>GGSMSNPDYCIPNFSQTVNERTIIDIFTICRYRSPLVVFCLSHNELAKKYAQDVSMSSGTHVHIIDGSVEITVSLYRTFRTIATQLLGRMQIVVFVTVDKSVVSTQVMKSIAWAFRGSFVELRNQSVDSSTLVSKLENLVSFAPLYNVPKCGPDYYGPTVYSELLSLATNARTHWYATIDYSMFTRSVLTGFVAKYFNEEAVPIDKRIVSIVGYNPPYVWTCLRHGIRPTYIEKSLPNPGGKGPFGLILPVINELVLKSKVKYVMHNPQIKLLCLDTFMLSTSMNILYIGAYPATHLLSLQLNGWTILAFDPKITSDWTDAMAKATGAKVIGVSKEFDFKSFSVQANQLNMFQNSKLSVIDDTWVETDYEKFQSEKQAYFEWLIDRTSIDVRLISMKWNRSKDTSVSHLLALLPQPYGASIREMRAFFHKKGASDIKILAAETEKYMDDFTAMSVSDQINTQKFMHCMITTVGDALKMDLDGGRAVIASYSLSNSSNSKERVLKFLSDANKAKAMVVFGAPNTHRLAYAKKVGLVLDSAIKMSKDLITFSNPTGRRWRDYGYSQSELYDAGYVEITIDQMVAYSSDVYNGVGYFA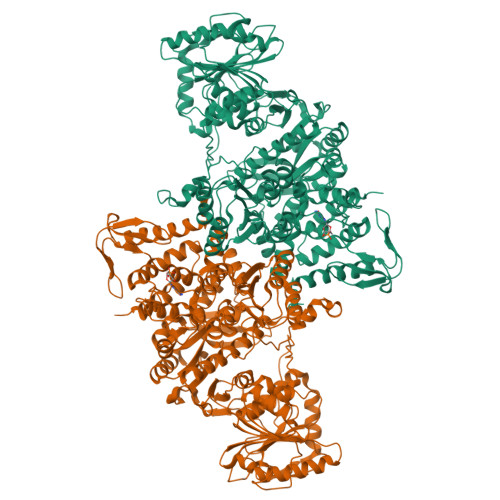NSTYNDLFSWYIPKWYVHKRMLMQDIRLSPAALVKCFTTLIRNICYVPHETYYRFRGILVDKYLRSKNVDPSQYSIVGSGSKTFTVLSHFEVPHECGPLVFEASTDVNISGHLLSLAIAAHFVASPMILWAEQMKYMAVDRMLPPNLDKSLFFDNKVTPSGALQRWHSREEVLLAAEICESYAAMMLNNKHSPDIIGTLKSAINLVFKI[2x]tert-butyl isocyanide | C5 H9 N | 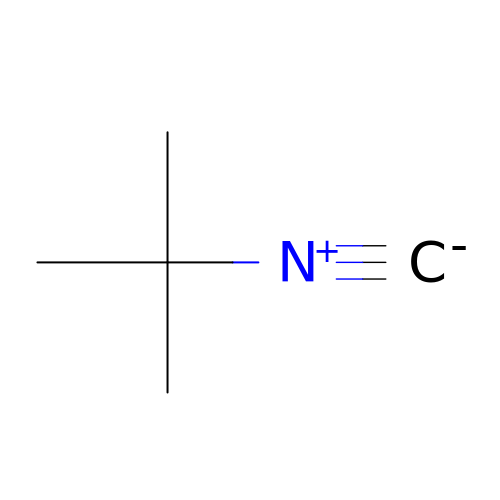FAGLEPBREOXSAC-UHFFFAOYSA-N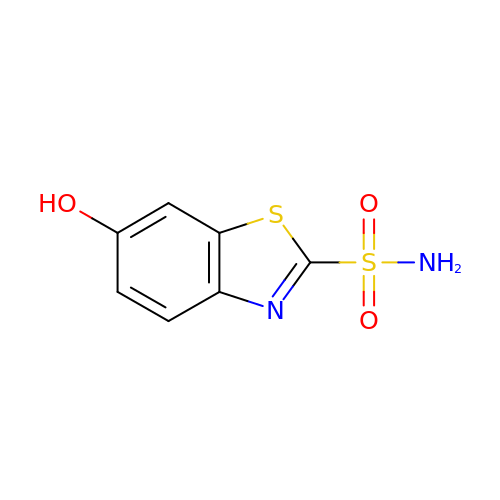6-HYDROXY-1,3-BENZOTHIAZOLE-2-SULFONAMIDE | C7 H6 N2 O3 S2 | NOOBQTYVTDBXTL-UHFFFAOYSA-N> MGATTQYTTLPSVLLIGPSGAGKTALLTLFERGPLLNPDGTSVGAADLKNPYRKPIVTSPVAQTHTSQVPTSVELAVGANEDGTPTSYKVDLD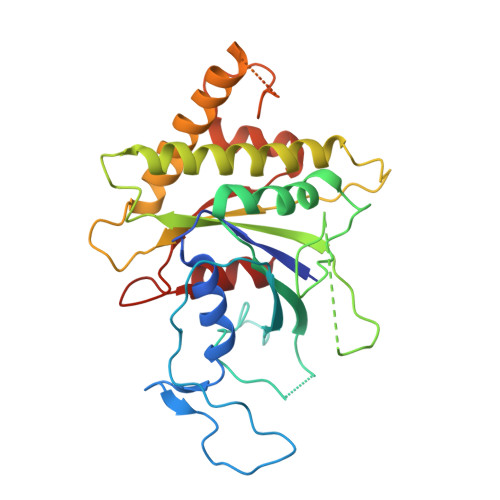AAGATARKFLLIDTPGHPKLRGTTLQHLLNPSPSLTIIPTNAPNKKTSTDSHSDPYKSKLKAVIFLLDAAALADSDGDYLSQTASYLYDVLLSLQKRFHSRKNSRAPSSIPVLIAANKQDLFTAVPASLVKSRLEHELGRIRKTRQKGLLEASVTSEDEIRADDEEGWLGAVGSKEFKFEEMMEFDMEVEVMGGNVIGDGPGAERWWRWIGERI>[2x]GPMGQKGWKFQGEQGEFRLEQPEHNSYLYFPLVNEAGMMSAVTP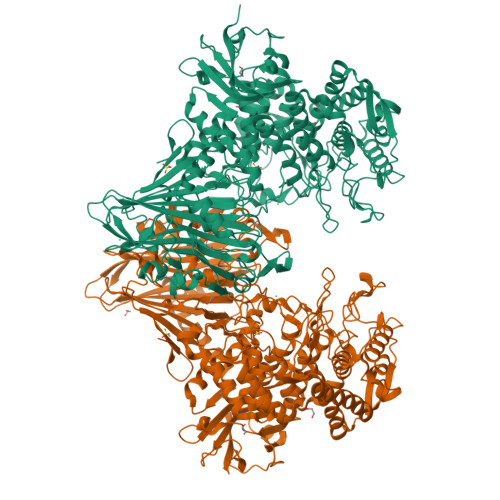NLHGEITSGHNTFLMEPVSAESLHNSKASRNFWVFIEGYGAWSVSGNSARQNAARFTGEEERSAVEAGFLWHAVTRENEKAGLKARTVSFVPVTDDKIELMRVTLTNTGNAPLKLTPTAAIPLYGRSADDLRDHRHVTSLLHRIFTSEYGIEVQPALSFDERGHRVNKVTYGVFGAEAGGTAPAGFFPVTEDFIGEGGALDWPEAVVANREPDAQAGTAVEGYEAVGALRFAPVELAPGKSVSYVVAMVISGDRIDVGRYAADYLAAGRFDALLEQNRAYWRDKLDTVRFSSGDGEQDLWMKWVTLQPILRRLYGNSFLPYHDYGRGGRGWRDLWQDCLALMVMEPAEVRHLLLNNYAGVRMDGSNATIIGAGPGEFVADRNNIPRVWMDHGAWPLMTTLLYLHQSGDLDLLFQPQSYFRDVFVKRCRERDASWTPEQGNKLLTADGQIYEGTILEHILLQNIVPFFNVGEHGNIKLEGADWNDGLDLAPERGESVAFTAFYASNLMELSELLLELQKRTGKDSLDIAEEMALLLDTLGKPISYDSIQEKRSLLDRYYDAVTPRVSGKKLLLDIRKVAEDLKRKADWAVAHLRGSEWIQSKEGYAWFNGYYNNDGERVEGDHPDGVRMTLTGQVFAIMGGVATDEQTEKISQAVNRYLKDERIGYRLNSRFGGIQQNLGRAFGFAFGHKENGAMFSHMTVMYANALYKRGFVQEGFEVLDSIYRLSADFENSRIYPGVPEYINERGRGMYTYLTGSASWLLLTQLTEVYGVKGRFGDLRLEPKLVQAQFDGSGEAAVETLFAGRMLRVVYRNPQAAEHGQYRVDSVSLNGQSVDCQNDGAGCLIGRSLIEALPADGVHELIVTLGRNIS>AASEDEFLRYLWRDYLYPKQYAWVLIAAYVAVFVVALVGNTLVCLAVWRNHHMRTVTNYFLVNLSLADVLATAICLPASLLVDITESWLFGHALCKVIPYLQAVSVSVAVLTLSFIALDRWYAICHPLLFKSTARRALGSILG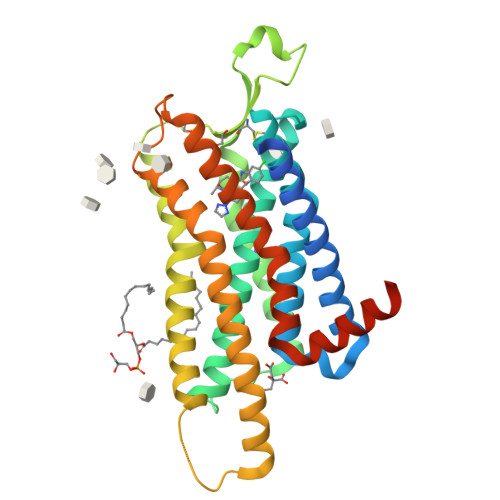IWAVSLAIMVPQAAVMECSSVLPELAARTRAFSVCDERWADDLAPKIYHSCFFIVTYLAPLGLMAMAYFQIFRKLWGRQIPGTTSAEVKQMRARRKTAKMLMVVVLVFALCYLPISVLNVLKRVFGMFRQASDREAVYAAFTFSHWLVYANSAANPIIYNFLSGKFREQFKAAFSWWLPGLAAAHHHHHHHHH[2x]>ETLVRPKPLLLKLLKSVGAQKDTYTMKEVLFYLGQYIMTKRLYDEKQQHIVYCSNDLLGDLFGVPSFSVKEHRKIYTMIYRN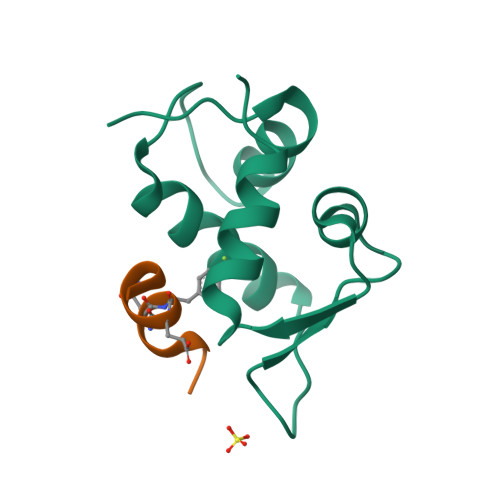LVV[3x];>[3x]TAWYANXEKLLR>MTYKIMAINAGSSSLKFQLLNMPQGALLCQGLIERIGLPEARFTLKTSAQKWQETLPIADHHEAVTLLL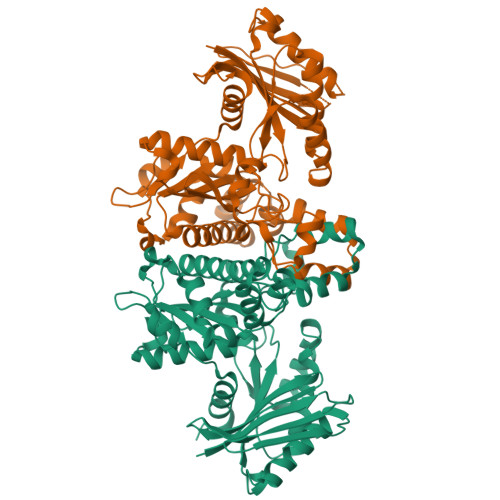EALTGRGILSSLQEIDGVGHRVAHGGERFKDAALVCDDTLREIERLAELAPLHNPVNALGIRLFRQLLPAVPAVAVFDTAFHQTLAPEAWLYPLPWRYYAELGIRRYGFHGTSHHYVSSALAEKLGVPLSALRVVSCHLGNGCSVCAIKGGQSVNTSMGFTPQSGVMMGTRSGDIDPSILPWLVEKEGKSAQQLSQLLNNESGLLGVSGVSSDYRDVEQAADAGNERAALALSLFAERIRATIGSYIMQMGGLDALIFTGGIGENSARARAAICRNLHFLGLALDDEKNQRSATFIQADNALVKVAVINTNEELMIARDVMRLALPQARELAVSA[2x]>[2x]MSFEEFTPLNEKSLVDYIKSTPALSSKIGADKSDDDLVIKEVGDGNLNFVFIVVGSSGSLVIKQALPYIRCIGESWPMTKERAYFEATTLRKHGNLSPDHVPEVYHFDRTMALIGMRYLEPPHIILRKGLIAGIEYPFLADHMSDYMAKTLFFTSLLYHDTTEHRRAVTEFCGNVELCRLTEQVV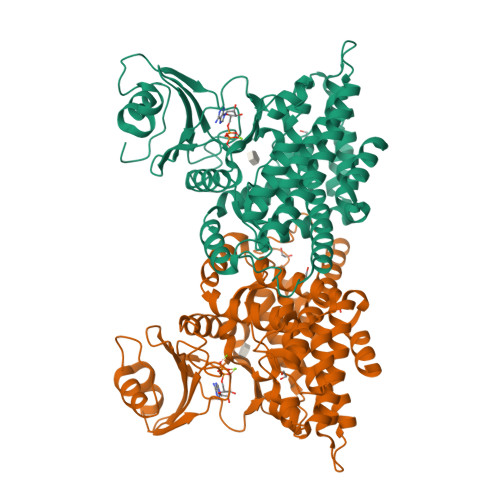FSDPYRVSTFNRWTSPYLDDDAKAVREDSALKLEIAELKSMFCERAQALIHGDLHTGSVMVTQDSTQVIDPEFSFYGPMGFDIGAYLGNLILAFFAQDGHATQENDRKEYKQWILRTIEQTWNLFNKRFIALWDQNKDGPGEAYLADIYNNTEVLKFVQENYMRNLLHDSLGFGAAKMIRRIVGVAHVEDFESIEEDKRRAICERSALEFAKMLLKERRKFKSIGEVVSAIQQQS>[4x]MRNKIFISHATPDDNDFTRWLALKLIGLGYEVWCDILFLDKGVDFWSNIEKVIREDTCKFLLVSSSYSNQREGVLKELAVAAKVKKQLKDDKFIIPLAIDEQLSYDDINIDIVRLNAIDFKMSWARGLKDILEAFEKQKVPKEVADASKSNLLYQQIFLHDKSVIEKEEIYDSNWLSILSFPEELRFHEYNWMLPKRFDVRELTFPAVRYKNYLCTFAWAYDFTYHLPKTETYHKSKTIRIPTEEILSGSYDSNFIRNAECKRLIVQLLNKAFELRMKDKEVQEYEMSNKTAYWLEKGKLEKDKFEKTMLVGKQKDKNWHFAISGASKLYPFPVLMISSHIFFTADGKKLIDSSSVQHSSRRRQGKNWWNN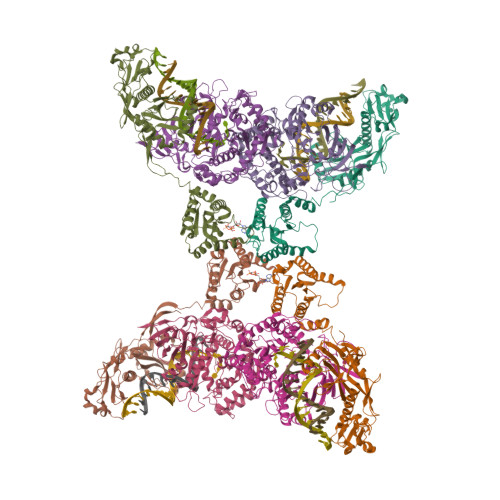TWRTKLLAFIKYLSDDDTSFYLEMGSEEKVFVSNEPVKFKGNVSYNIPEKNTLEEEAELSGFNQGEDIEELEELIENLEAE;>[4x]MKELIYIEEPKILFAHGQKCTDARDGLALFGPLNNLYGIKSGVIGTKQGLKIFRDYLDHIQKPIYNSNSITRPMFPGFEAVFDCKWESTGITFKEVTNEDIGKFLYNSSTHKRTYDLVSLFIDKIISANKNEDENVDVWFVIVPDEIYKYCRPNSVLPKEMVQTKALMSKSKAKSFRYEPSLFPDINIELKEQEKEAETYNYDAQFHDQFKARLLKHTIPTQIFRESTLAWRDFKNAFGLPIRDFSKIEGHLAWTISTAAFYKAGGKPWKLSDVRNGVCYLGLVYKKVEKSKNPRNACCAAQMFLDNGDGTVFKGEVGPWYNPKNGQYHLEPKEAKALLSQSLQSYKEQIGEYPKEVFIHAKTRFNHQEWDAFLEVTPKETNLVGVTISKTKPLKLYKTEGDYTILRGNAYVVNERSAFLWTVGYVPKIQTALSMEVPNPLFIEINKGEADIKQVLKDILSLTKLNYNACIFADGEPVTLRFADKIGEILTASTDIKTPPLAFKYYI>[3x]GASNSYA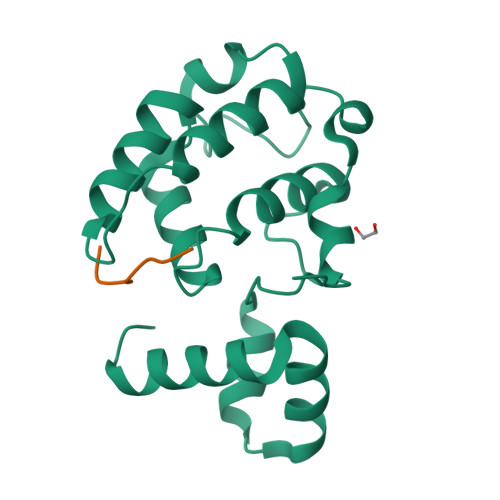IPENELLDEDTMNFISSLKNDLSNISNSLPFEYPHEIAEAIRSDFSNEDIYDNIDPDTISFPPKIATTDLFLPLFFHFGSTRQFMDKLHEVISGDYEPSQAEKLVQDLCDETGIRKNFSTSILTCLSGDLMVFPRYFLNMFKDNVNPPPNVPGIWTHDDDESLKSNDQEQIRKLVKKHGTGRMEMRKRFFEKDLL;>[3x]ADISVLPEIRIPIFNSLKMQ>[4x]MKRSLRKMWRPGEKKEPQGVVYEDVPDDTEDFKESLKVVFEGSAYGLQNFNKQKKLKRCDDMDTFFLHYAAAEGQIELMEKITRDSSLEVLHEMDDYGNTPLHCAVEKNQIESVKFLLSRGANPNLRNFNMMAPLHIAVQGMNNEVMKVLLEHRTIDVNLEGENGNTAVIIACTTNNSEALQILLKKGAKPCKSNKWGCFPIHQAAFSGSKECMEIILRFGEEHGYSRQLHINFMNNGKATPLHLAVQNGDLEMIKMCLDNGAQIDPVEKGRCTAIHFAATQGATEIVKLMISSYSGSVDIVNTTDGCHETMLHRASLFDHHELADYLISVGADINKIDSEGRSPLILATASASWNIVNLLLSKGAQVDIKDNFGRNFLHLTVQQPYGLKNLRPEFMQMQQIKELVMDEDNDGCTPLHYACRQGGPGSVNNLLGFNVSIHSKSKDKKSPLHFAASYGRINTCQRLLQDISDTRLLNEGDLHGMTPLHLAAKNGHDKVVQLLLKKGALFLSDHNGWTALHHASMGGYTQTMKVILDTNLKCTDRLDEDGNTALHFAAREGHAKAVALLLSHNADIVLNKQQASFLHLALHNKRKEVVLTIIRSKRWDECLKIF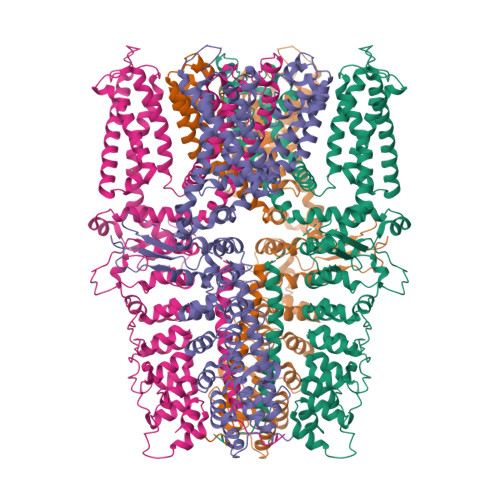SHNSPGNKCPITEMIEYLPECMKVLLDFCMLHSTEDKSCRDYYIEYNFKYLQCPLEFTKKTPTQDVIYEPLTALNAMVQNNRIELLNHPVCKEYLLMKWLAYGFRAHMMNLGSYCLGLIPMTILVVNIKPGMAFNSTGIINETSDHSEILDTTNSYLIKTCMILVFLSSIFGYCKEAGQIFQQKRNYFMDISNVLEWIIYTTGIIFVLPLFVEIPAHLQWQCGAIAVYFYWMNFLLYLQRFENCGIFIVMLEVILKTLLRSTVVFIFLLLAFGLSFYILLNLQDPFSSPLLSIIQTFSMMLGDINYRESFLEPYLRNELAHPVLSFAQLVSFTIFVPIVLMNLLIGLAVGDIADVQKHASLKRIAMQVELHTSLEKKLPLWFLRKVDQKSTIVYPNKPRSGGMLFHIFCFLFCTGEIRQEIPNADKSLEMEILKQKYRLKDLTFLLEKQHELIKLIIQKMEIISETEDDDSHCSFQDRFKKEQMEQRNSRWNTVLRAVKAKTHHLEP> HVRSESSVENFLSRSACVYIVEYKTRDDTPDKMYDSWV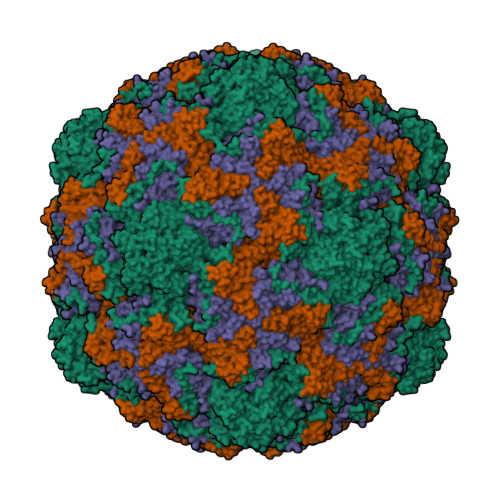INTRQVAQLRRKLEFFTYVRFDVEVTFVITSVQDDSTRQNTDTPALTHQIMYVPPGGPIPQAVDDYNWQTSTNPSVFWTEGNAPPRMSIPFMSVGNAYSNFYDGWSHFSQTGVYGFNTLNNMGKLYFRHVNDKTISPITSKVRIYFKPKHVKAWVPRPPRLCEYTHKDNVDFEPKGVTTSRTQLTISNS;> SDRVRSITLGNSTITTQESANVVVGYGVWPDYLSDEEATAEDQPTQPDVATCRFYTLDSVSWMKESQGWWWKFPDALRDMGLFGQNMQYHYLGRSGYTIHVQCNASKFHQGCLLVVCVPEAEMGAANINEKINREHLSNGEVANTFSGTKSSNTNDVQQAVFNAGMGVAVGNLTIFPHQWINLRTNNCATIVMPYINSVPMDNMFRHYNFTLMIIPFAKLDYAAGSSTYIPITVTVAPMCAEYNGLRLG;> GLPVMNTPGSNQFLTSDDYQSPTAMPQFDVTPEMNIPGEVKNLMEIAEVDSVVPVNNVNENVNSLEAYRIPVHSVTETGAQVFGFTLQPGADTVMERTLLGEILNYYANWSGSIKLTFMYCGSAMATGKFLLAYSPPGAGVPKNRREAMLGTHIIWDIGLQSSCVLCVPWISQTHYRFVSKDSYTDAGFITCWYQTSIVVPAEVQNQSVILCFVSACNDFSVRLLRDSPFVRQT> CPRGVYVNFYSQTECAENPSYPAEVARLNVYAFDKDGILRSANVFEDVQLSAAKEWLIPLEKDGLYTIFAWGNIDDHYNIGEIKIGETTKQQVLMRLKQDGKWATNIDGTTLWYATSPVVELKNMEDGADQYIHTRANLREYTNRVTVSVDSLPHPENYEIKLASSNGSYRFDGTVAKADSTYYPGETKVVGDSTCRAFFTTLK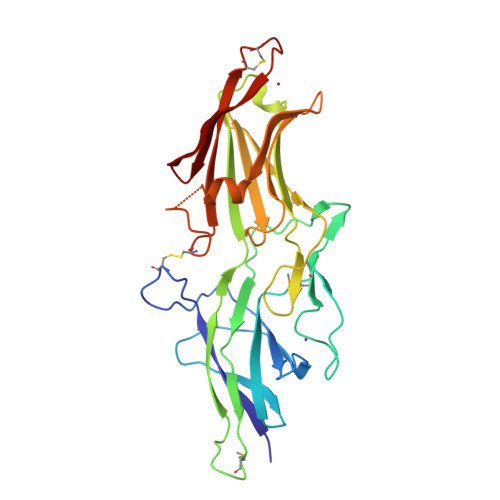LESGHENTLSVTHKPTGREIFRTDLVGAILSSQYAQNINLRCINDFDIRLVAHHCNCPDDTYVVVQIWINGWLIHSY N'-{(1S,2S)-1-(3,5-difluorobenzyl)-2-hydroxy-2-[(2R)-4-(phenylcarbonyl)piperazin-2-yl]ethyl}-5-methyl-N,N-dipropylbenzene-1,3-dicarboxamide | C35 H42 F2 N4 O4 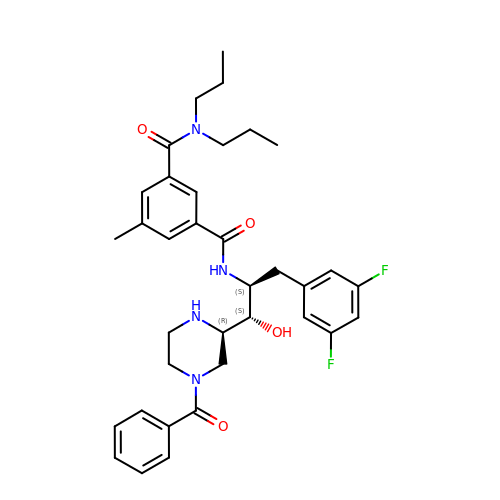| ZJLWDMHHAMNWRK-QAXCHELISA-N> GSMENTDVFLGLHDFLERMRKPSAGDFVKSIKSFIVSFSNNAPDPEKDCAMVQEFF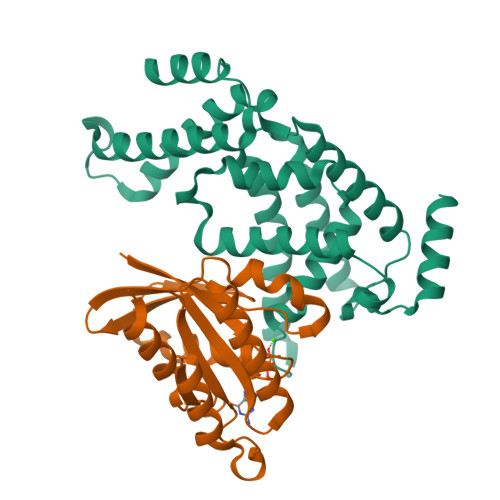SKMEAAFRAHPLWSGCSEEELDSAGDGLEKYVMTKLFTRVFASNTEEVIADEKLFQKMSLVQQFISPENLDIQPTFQNESSWLLAQKELQKINMYKAPRDKLVCILNCCKVINNLLLNASIASNENAPGADEFLPVLIYVTIKANPPQLHSNLLYIQRYRRESKLVGEAAYFFTNILSAESFISNIDAKSISLDEAEFEKNMESARARISG;> GSMAAAGNKSINAKLVLLGDVGAGKSSLVLRFVKDQFVEFQESTIGAAFFSQTLAVNDATVKFEIWDTAGQERYHSLAPMYYRGAAAAIIVFDVTNQASFERAKKWVQELQAQGNPNMVMALAGNKSDLLDARKVTAEDAQTYAQENGLFFMETSAKTATNVKEIFYEIARRLPRVQPTEN> HMTPPKAEKRPYPITTHGDTRVDDYYWLRDDERTDPQVLDYLQAENAFTDAALKPQQALRETLYEEMVARENLYFQSVPYVRHGYRYQTRFEPGNEYAIYVRQPQAESEHWDTLIDGNQRAEQREFYTLGGLEVSPDNQKLAVAEDFLSRRQYDIRFKNLSDDSWTDEVLENTSGSFEWANDSATVYYVRKHAKTLLPYQVYRHVVGTDPQLDELIYEEQDDTFYVGLEKTTSDRFILIHLSSTTTSEILLLDADRADSTPQMFVPRRKDHEYGIDHYHQHFYIRSNKDGKNFGLYQSEQADEAQWQTLIAPRIEVMLEGFSLFRDWLVVEERSEGLTQLRQIHWQSGEVKRIAFDDPTYTTWLAYNPEPETELLRYGYSSMTTPTTLYELNLDSDERVMLKQQEVKNFTPENYRSERVWVKARDGVEVPVSLVYRHDSFARGTNPLMVYGYGSYGSSMDPAFSASRLSLLDRGFVFVLAHIRGGGELGQLWYEDGKLFKKQNTFNDFIDVTEALIAQGY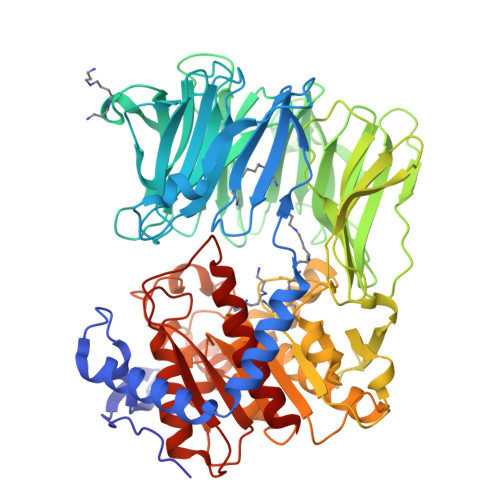GDAKRVFAMGGSAGGLLMGAVINQAPELFNGIVAQVPFVDVVTTMLDESIPLTTGEYDEWGNPNQQAYYDYILQYSPYDQVKAQDYPHMLVTTGLHDSQVQYWEPAKWVAKLRELKTDDRQLLLYTDMDSGHGGKSGRFKAYEDIALEYAFILALAE> GSLILEREEEIRNIEQGVSDLNVLFQQVAQLVAEQGEVLDTI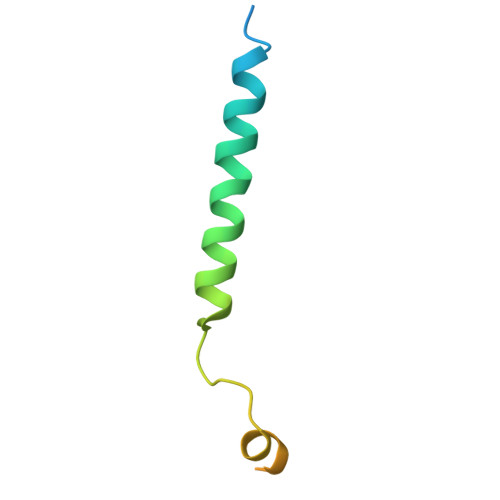ERNVEAVGDDTRGADRELRAAARYQ>[5x]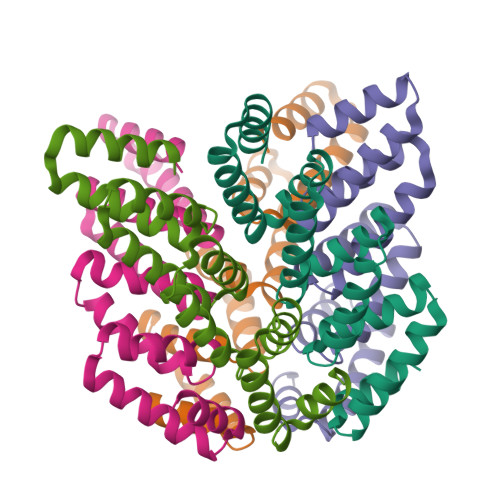MVEELKRKLRQAKEDGDEELLERVKNEMLLLAVVDPRVLVEVLNTAKELGDEEMYKKVKGIMLRLAVVDPRVLVLVLELAEALGDEEMKEKVKNIMLLLAVVDPRVLVLVLELAEELGDEEMKKEVEEILDKLAEVDPRVAVLKEVAKKEGSWLEHHHHHH5-ethyl-4-fluoro-2-[(2-methylpyridin-3-yl)oxy]phenol | C14 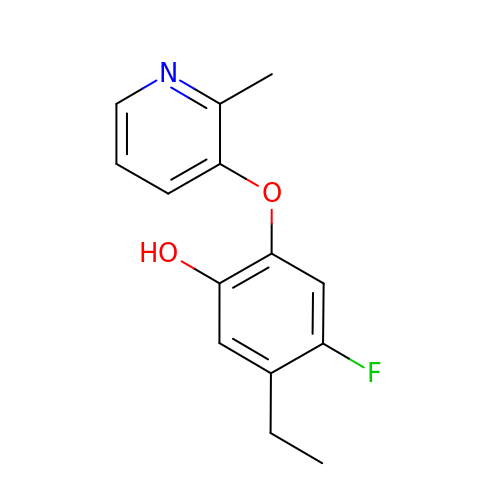H14 F N O2 | VHXDJFGLVVJBNS-UHFFFAOYSA-N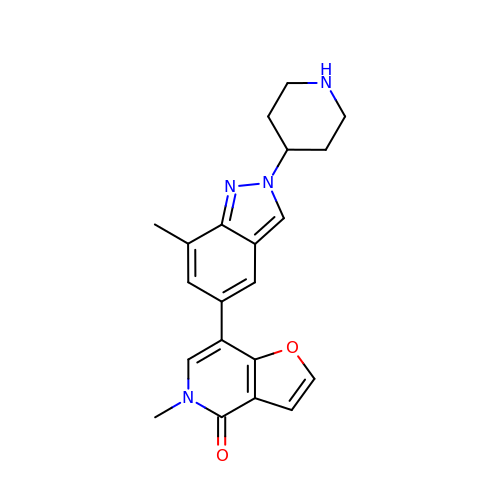5-methyl-7-(7-methyl-2-piperidin-4-yl-indazol-5-yl)furo[3,2-c]pyridin-4-one | C21 H22 N4 O2 | ZDDPECPWLZOLGO-UHFFFAOYSA-N> MAMM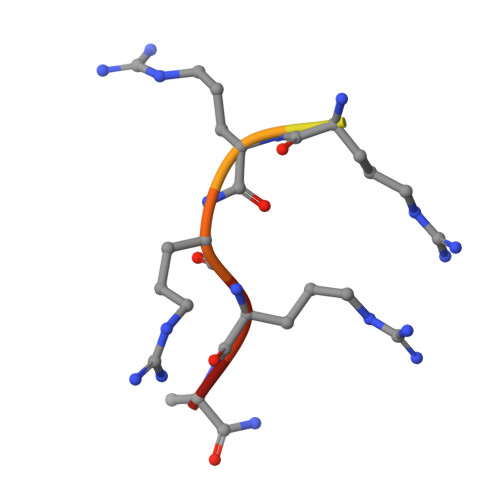XRRRRAX> MGKALVIVESPAKAKTINKYLGSDYVVKSSVGHIRDLPTSGSAAKKSADSTSTKTAKKPKKDERGALVNRMGVDPWHNWEAHYEVLPGKEKVVSELKQLAEKADHIYLATNLDREGEAIAWHLREVIGGDDARYSRVVFNEITKNAIRQAFNKPGELNIDRVNAQQARRFMDRVVGYMVSPLLWKKIARGLSAGRVQSVAVRLVVEREREIKAFVPEEFWEVDASTTTPSGEALA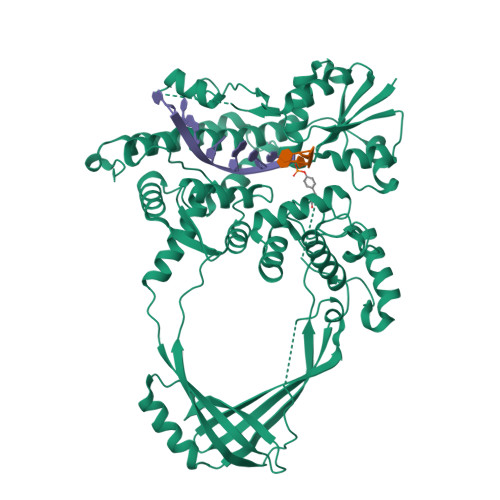LQVTHQNDKPFRPVNKEQTQAAVSLLEKARYSVLEREDKPTTSKPGAPFITSTLQQAASTRLGFGVKKTMMMAQRLYEAGYITYMRTDSTNLSQDAVNMVRGYISDNFGKKYLPESPNQYASKENSQEAHEAIRPSDVNVMAESLKDMEADAQKLYQLIWRQFVACQMTPAKYDSTTLTVGAGDFRLKARGRILRFDGWTKVMPALRKGDEDRILPAVNKGDALTLVELTPAQHFTKPPARFSEASLVKELEKRGIGRPSTYASIISTIQDRGYVRVENRRFYAEKMGEIVTDRLEENFRELMNYDFTAQMENSLDQVANHEAEWKAVLDHFFSDFTQQLDKAEKDPEEGGMRPNQMVLT>DAPVPVPVPVPVPVAVSGATTAGLRAQAARLAGHLRERPALGPEAVARPLLLSRAQRERRAVVVAADRDSLLTGLDALAGGEAGPRLASGAADVTGRVVLVFPGQGAHWTGVAERLWREAPVFADSMARCADVLRDLAGWELREVLVDPVALERVDVLQPVSFAVVVSLAALWASVGVRPDAVVGHSQGEVAAAHVAGALTLAEAARIVVLRSALIARELSGRGAMLTVVADVERVTALLAGFEGRVCVAAVNGPASVTVSGEDGAVREFERVLSARRMLRWRLPGVDFAGHSPQVDALRAELLAALGDIASREPEIPLLSTVTGEPATRLDAEHWYRNLREPVRFADAVTALLDRGHRV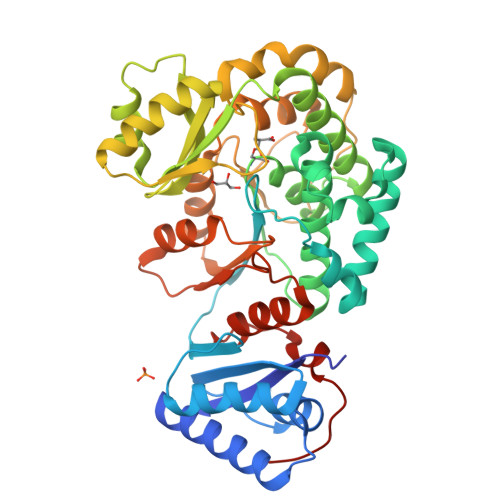FVEVSPHPVLTTSVVDLAAPHRTAVVGTLRRDEGGLDRFLLSAAELHVRGVPVDLARHAGAGTAEVPTTVFQ[4x]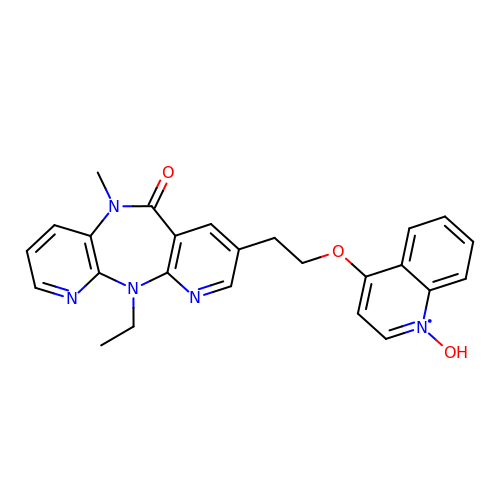11-ethyl-5-methyl-8-[2-(1-oxidanylquinolin-4-yl)oxyethyl]dipyrido[3,2-[1,4]diazepin-6-one | C25 H24 N5 O3 | PQGWYSJEHPHRGI-UHFFFAOYSA-N>[2x]MKDKVRAMRSLLISDEFAGLKNAIDRFMLILSTLHRID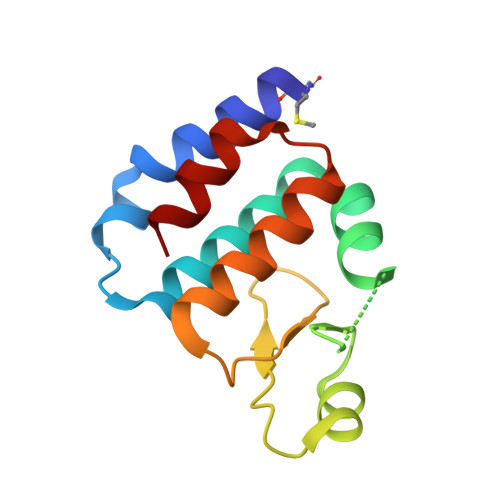SASFSEATMFKGRKRVYFADNEQTLLASGQTTKPKAIPNTPFWVITNNNTSRKQQMVEQVMVRMGFPSDIIEKVTHSI> SNAGKKSRVKTQKSGTGATATVSPKEILNLTSELLQKCSSPAPGPGKEWEEYVQIRTLVEKIRKKQKGLSVTFDGKREDYFPDLMKWASENGASVEGFEMVNFKEEGF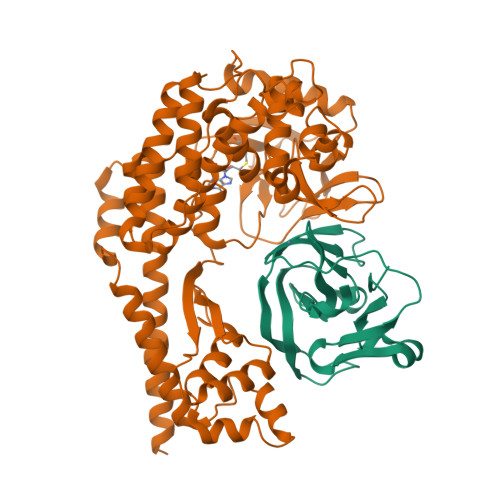GLRATRDIKAEELFLWVPRKLLMTVESAKNSVLGPLYSQDRILQAMGNIALAFHLLCERASPNSFWQPYIQTLPSEYDTPLYFEEDEVRYLQSTQAIHDVFSQYKNTARQYAYFYKVIQTHPHANKLPLKDSFTYEDYRWAVSSVMTRQNQIPTEDGSRVTLALIPLWDMCNHTNGLITTGYNLEDDRCECVALQDFRAGEQIYIFYGTRSNAEFVIHSGFFFDNNSHDRVKIKLGVSKSDRLYAMKAEVLARAGIPTSSVFALHFTEPPISAQLLAFLRVFCMTEEELKEHLLGDSAIDRIFTLGNSEFPVSWDNEVKLWTFLEDRASLLLKTYKTTIEEDKSVLKNHDLSVRAKMAIKLRLGEKEILEKAVKSAAVNREYYRQQMEEKAPLPKYEESNLGLLESSVGDSRLPLVLRNLEEEAGVQDALNIREAISKAKATENGLVNGENSIPNGTRSENESLNQESKRAVEDAKGSSSDSTAGVKE;> SNAMGQQSGAVYVGNYRVVNRHLATSADWQNCVWESYNRDLLVSTTTAHGCDIIARCQCTTGVYFCASKNKHYPISFEGPGLVEVQESEYYPRRYQSHVLLAAGFSEPGDAGGILRCEHGVIGIVTMGGEGVVGFADIRDLLWLEDDAMEQ> GSHMSVAQVATGSPRPGLFHLDSSVVDLSGDDFSRVHRVAPLCPWIVLFYNDGCGACRRYASTFSKFAGGLKVEHGKDALQIATAAAVNCASEVDLC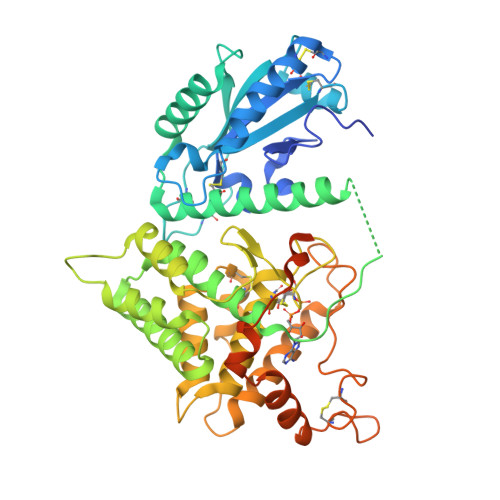RKYDINFVPRLFFFYPRDSCRSNEECGTSSLEHVAFENSHLEVDELESEVRRLVNKHMVVDDSLKERCIDMHFKLYTSKEELVKRSVSSTDESGRFVETTELYATDIAGAFFSAMHYDVSLVGTEPRERLTALEDFVLLVKDSLPSIGADGVVSALESITAERPFTVASWQDAVVKSGIPFDGSPRNVRWRTCRGSSPQYRGFPCGMWLLLHALTVNTPADRNVLEVIQNYIRYFFSCKECRDHFIQFNFSPNEDPVLQLWRAHNNVNARLANVKDGADPLVPKRQFPTLEACTECYDGAGNFIEAHVTGFLKQRYLWDPKAVGLMESNDDLNEVDPASKDANVGRNVESSGKGKGDGGARGNSKEVRSDHAG> MSFESKKPMRTWSHLAEMRKKPSEYDIVSRKLHYSTNNPDSPWELSPDSPMNLWYKQYRNASPLKHDNWDAFTDPDQLVYRTYNLMQDGQESYVQSLFDQFNEREHDQMVREGWEHTMARCYSPLRYLFHC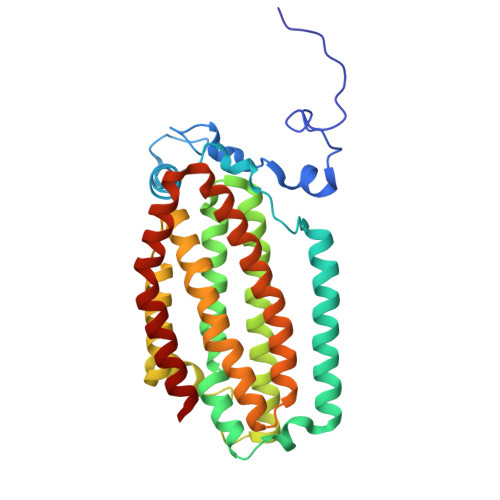LQMSSAYVQQMAPASTISNCCILQTADSLRWLTHTAYRTHELSLTYPDAGLGEHERELWEKEPGWQGLRELMEKQLTAFDWGEAFVSLNLVVKPMIVESIFKPLQQQAWENNDTLLPLLIDSQLKDAERHSRWSKALVKHALENPDNHAVIEGWIEKWRPLADRAAEAYLSMLSSD> ACGYSDRVLQLTLGNSTITTQEAANSVVAYGRWPEFIRDDEANPVDQPTEPDVATCRFYTLDTVMWGKESKGWWWKLPDALRDMGLFGQNMYYHYLGRSGYTVHVQCNASKFHQGALGVFAIPEYCLAGDSDKQRYTSYANANPGERGGKFYSQFNKDNAVTSPKREFCPVDYLLGCGVLLGNAFVYP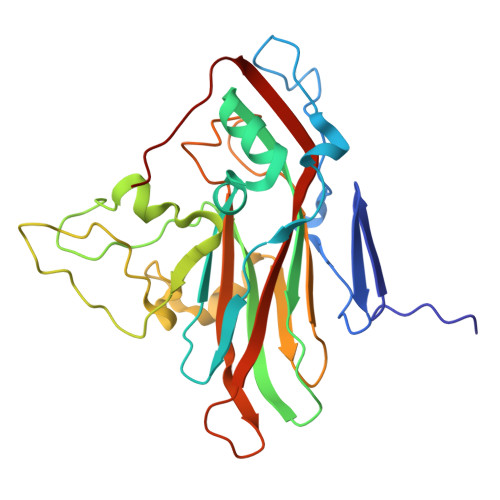HQIINLRTNNSATIVLPYVNALAIDSMVKHNNWGIAILPLSPLDFAQDSSVEIPITVTIAPMCSEFNGLRNVTAPKFQ> SSSF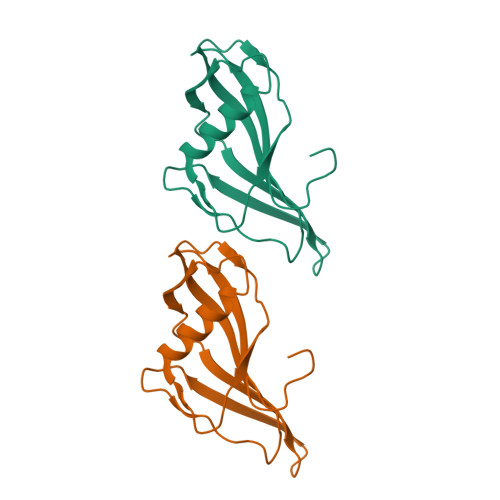DKGKYKKGDDASYFEPTGPYLMVNVTGVDGKGNELLSPHYVEFPIKPGTTLTKEKIEYYVEWALDATAYKEFRVVELDPSAKIEVTYYDKNKKKEETKSFPITEKGFVVPDLSEHIKNPGFNLITKVVIEKK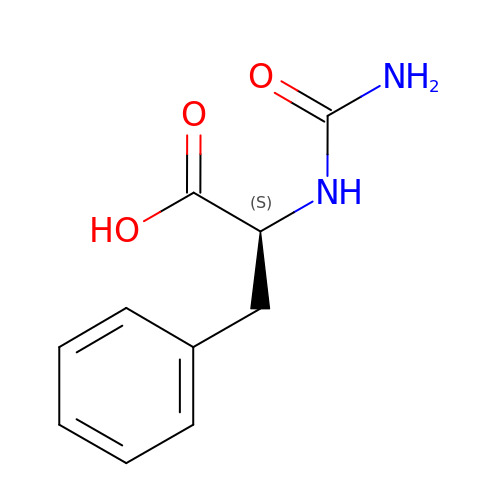D-[(AMINO)CARBONYL]PHENYLALANINE | C10 H12 N2 O3 | IPWQOZCSQLTKOI-QMMMGPOBSA-N>[2x]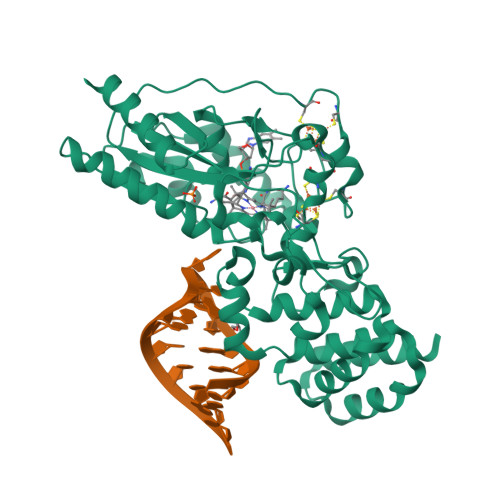MASRGSHHHHHHGAGDRGPEFELGTRGSMNVYQLKEELIEYAKSIGVDKIGFTTADTFDSLKDRLILQESLGYLSGFEEPDIEKRVTPKLLLPKAKSIVAIALAYPSRMKDAPRSTRTERRGIFCRASWGKDYHDVLREKLDLLEDFLKSKHEDIRTKSMVDTGELSDRAVAERAGIGFSAKNCMITTPEYGSYVYLAEMITNIPFEPDVPIEDMCGSCTKCLDACPTGALVNPGQLNAQRCISFLTQTKGFLPDEFRTKIGNRLYGCDTCQTVCPLNKGKDFHLHPEMEPDPEIAKPLLKPLLAISNREFKEKFGHVSGSWRGKKPIQRNAILALAHFKDASALPELTELMHKDPRPVIRGTAAWAIGKIGDPAYAEELEKALEKEKDEEAKLEIEKGIELLKASGMTKQGLSGSLEVDLQGDHGLSAWSHPQFEK>CSLIPDYQRPEAPVAAAYPQGQAYGQNTGAAAVPAADIGWREFFRDPQLQQLIGVALENNRDLRVAALNVEAFRAQYRIQRADLFPRIGVDGSGTRQRLPGDLSTTGSPAISSQYGVTLGTTAWELDLFGRLRSLRDQALEQYLATEQAQRSAQTTLVASVATAYLTLKADQAQLQLTKDTLGTYQKSFDLTQRSYDVGVASALDLRQAQTAVEGARATLAQYTRLVAQDQNALVLLLGSGIPANLPQGLGLDQTLLTEVPAGLPSDLLQRRPDILEAEHQLMAANASIGAARAAFFPSISLTANAGTMSRQLSGLFDAGSGSWLFQPSINLP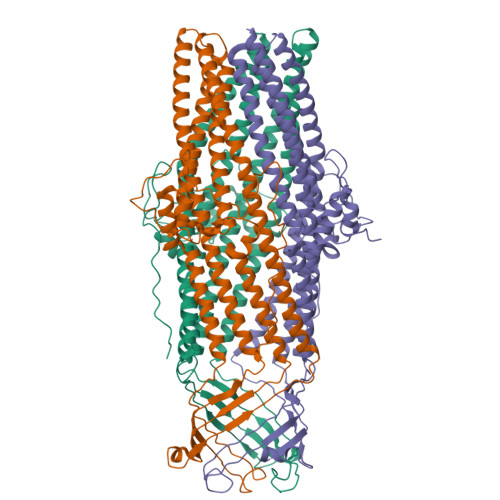IFTAGSLRASLDYAKIQKDINVAQYEKAIQTAFQEVADGLAARGTFTEQLQAQRDLVKASDEYYQLADKRYRTGVDNYLTLLDAQRSLFTAQQQLITDRLNQLTSEVNLYKALGGGWNQQTVTQQQTAKKEDPQAHHHHHH[2x]>MSRQSISLRFPLLLLLLSPSPVFSADPGAPAPVNPCCYYPCQHQGICVRFGLDRYQCDCTRTGYSGPNCTIPEIWTWLRTTLRPSPSFIHFLLTHGRWLWDFV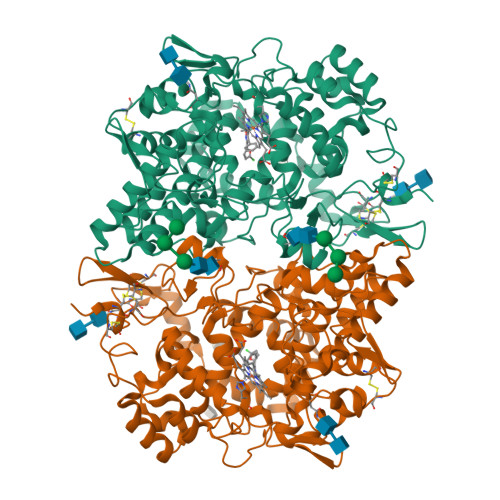NATFIRDTLMRLVLTVRSNLIPSPPTYNIAHDYISWESFSNVSYYTRILPSVPRDCPTPMDTKGKKQLPDAEFLSRRFLLRRKFIPDPQSTNLMFAFFAQHFTHQFFKTSGKMGPGFTKALGHGVDLGHIYGDNLERQYQLRLFKDGKLKYQMLNGEVYPPSVEEAPVLMHYPRGIPPQSQMAVGQEVFGLLPGLMLYATIWLREHNRVCDLLKAEHPTWGDEQLFQTARLILIGETIKIVIEEYVQQLSGYFLQLKFDPELLFGAQFQYRNRIAMEFNQLYHWHPLMPDSFRVGPQDYSYEQFLFNTSMLVDYGVEALVDAFSRQPAGRIGGGRNIDHHILHVAVDVIKESRVLRLQPFNEYRKRFGMKPYTSFQELTGEKEMAAELEELYGDIDALEFYPGLLLEKCHPNSIFGESMIEMGAPFSLKGLLGNPICSPEYWKASTFGGEVGFNLVKTATLKKLVCLNTKTCPYVSFHVPDPRQEDRPGVERPPTEL[2x]> MGELRVGLEESELWLRFKELTNEMIVTKNGRRMFPVLKVNVSGLDPNAMYSFLLDFVAADNHRWKYVNGEWVPGGKPEPQAPSCVYIHPDSPNFGAHWMKAPVSFSKVKLTNKLNGGGQIMLNSLHKYEPRIHIVRVGGPQRMITSHCFPETQFIAVTAYQNEEITALKIKYNPFAKAFLDAKERSHHHHHH

Brachyury is a transcription factor that plays an essential role in tumour growth of the rare bone cancer chordoma and is implicated in other solid tumours. Brachyury (encoded by the TBXT gene, also formerly known as T) is the founding member of the family and was first identified in 19275. The DNA binding domain forms an immunoglobulin-like fold and contacts DNA via an unusual insertion of an α-helix into the minor groove. All T-box proteins recognize a common consensus sequence named the T-box binding element (AGGTGTGAAA) with family member-specific variations found in the preferences for repeats, orientations (inverted or tandem), and spacing of such repeats.

We have also obtained a crystal structure of WT brachyury (at 2.7 Å resolution) in complex with a single T-box binding element half-site oligo which allows us to directly compare binding interfaces and DNA distortions between single and palindromic sites. Contacts to the DNA are made via loops between strands A and B, c and c’, and two α-helices following on from strand G at the C-terminal end of the DNA binding domain.>[2x]GSVVIVGRIILSGKGGPITAYSQQTRGLLGCIITSLTGRDRNQV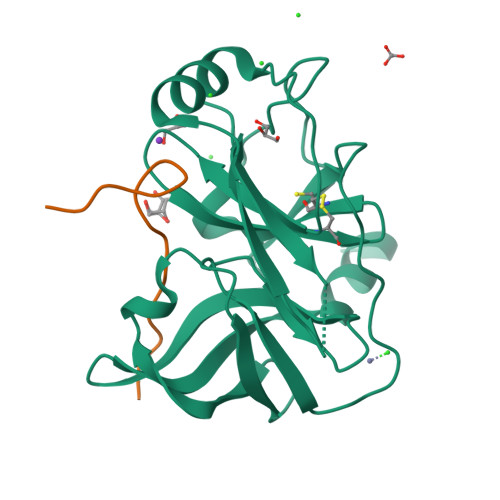EGEVQVVSTATQSFLATCVNGVCWTVYHGAGSKTLAGPKGPITQMYTNVDQDLVGWQAPPGARSLTPCTCGSSDLYLVTRHADVIPVRRRGDSRGSLLSPRPVSYLKGSSGGPLLCPSGHAVGIFRAAVCTRGVAKAVDFVPVESMETTMRGSHHHHHH;>GELGRLVYLLDGPGYDPIHCD[2x]> MKDIAIRGYCDRPSVATGETIRFYVSANETRGTFDAELVRLIHGDSNPAGPGYKEEAIKSDLEGQYPARFQRTQFGSYVEVADPDAGLQPDGAFSVHLFLWSTTPSRGRQGIASRWNDERQSGWNLAIEDGRVVFTIGDGSGATSSVVSDRPLFQQIWYSITGVYDPEKKQLRLYQKSVVNRTNSRFGLVVPLDSDCAVSADATVKAADSETSLLIAGLGEAAAQDGRTWCIAHYNGKVDAPKIYGCALGQDDAEKLSRGEIVRPISRLAHWDFSAGIGLNGIPTDHVVDASGYGHHGRCMNQPSRGSTGWNWDGHEENFIHCPEQYGALWFHEDCLDDCRWEKDFEFTVPEGLKSDFYAVKIRYEDTEDYIPFFVLPPRGTATAPILVIASTLSYLAYANEQIMHKADIGQAVAGHTPVLNENDVELHKNLSYYGLSTYDGHIDGRGVQYTSWRRPIMNLRPKHRQGFGSIWELPADLHLIDWLNHNGFEYDVATEHDLNDQGAELLRRYKVVLTGSHPAYQTWANADAWEDYLADGGRGMYLAANGMYWIVEVHPEKPWVMEVRKELGVTAWEAPPGEYHYSTNGRRGGRFRGRARATQKIWGTGMSSFGFDHSGYFVQMPDSQDERVAWIMEGIDPEERIGDGGLVGGGAGGYELDRYDLALGTPPNTLLLASSVEHSVVYT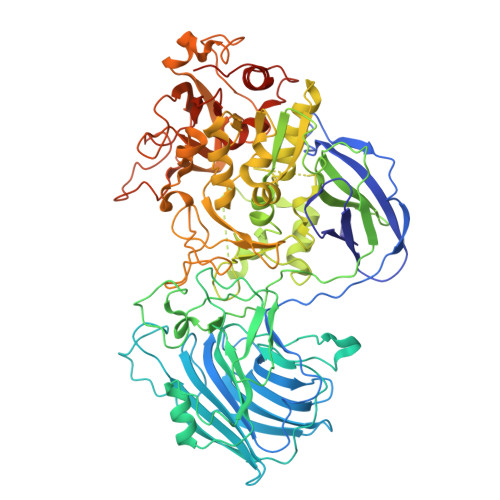VIPDDKAFPHPGMNGGEHPFVRADITYFSTANGGGMFATSSISWLGSLSWNDYDNNVSKMTKNVLNQFIKDEPAPRVKLAAALEHHHHHH> MDYTYADDSLTLHTDMYQINMMQTYWELGRADLHAVFECYFREMPFNHGYAIFAGLERLVNYLENLTFTESDIAYLREVEEYPEDFLTYLANFEFKCTVRSALEGDLVFNNEPLIQIEGPLAQCQLVETALLNMVNFQTLIATKAARIKSVIGDDPLLEFGTRRAQELDAAIWGTRAAYIGGADATSNVRAGKIFGIPVSGTHAHSLVQSYGNDYEAFMAYAKTHRDCVFLVDTYDTLKAGVPSAIRVAREMGDKINFLGVRIDSGDMAYISKRVREQLDEAGFTEAKIYASNDLDENTILNLKMQKSKIDVWGVGTKLITAYDQPALGAVFKLVSIEGEDGQMKDTIKLSSNAEKVTTPGKKQVWRITRKSDKKSEGDYVTLWNEDPRQEEEIYMFHPVHTFINKYVRDFEARPVLQDIFVEGKRVYELPTLDE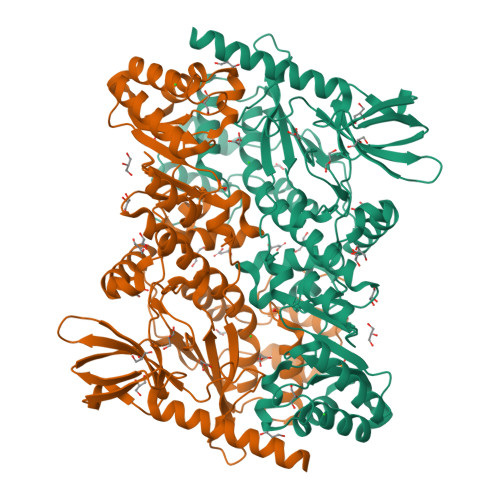IKQYAKENLDSLHEEYKRDLNPQKYPVDLSTDCWNHKMNLLEKVRKDVKHLTETVNKEA>MKTLLKNSLTFLLMLMPVLAFAQQAPQIMNVSARQTTSLDGQWKTIVDPFENGRGMKVYQDKTYSDKTKLQEYDFETDKLLFVPGDWNTQRPQLYYYEGTVWYRKHFEYSLQPGKRLFLNFGAVNYEAIVWLNGKRLGRHIGGFTPFNFEITNLLKEGTNSLVVKVDNKRLPEAVPTVNADWWNFGGITRPVTLIEMPATYIRDYYVQLAKDDKNMIEGWVQLEGSDKEQKITLDIPELKVKKEVTTDANGYASFLIKSKPILWTPENPKLYAVNLASETDKVSDEIGFRTIRTEGIKILLNDKEIFCRGISIHEETPYYSGRAYSKDHAHTLLSWAKELGCNFVRL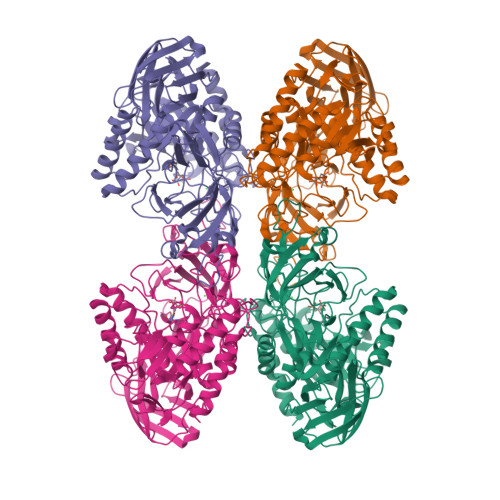AHYPHNEEMVREAERMGFLVWSEIPVYWTIHWENKDTYQNAEQQLCDMIARDKNRCNIIIWSIANETPHSKTRLTFLSNLANKARSLDSVRLIGAAMEKEEVQPGVLTVNDPLGELLDIISFNEYVGWYDGDSEKCDRVNWTFDTQKPVFISELGGGALYGHHGSPKERFTEEYQEDLYIRHVNMLKRIPGLAGTTPWILKDFRSPRRHVPEIQDDFNRKGLVSDKGQKKKAFFVLQKWYKELTEAYK[4x]>MFKTEFEFPEELKTKLQEHINYFPKKRQAILLCLHEIQNYYGYIPPESLKPLADMLELPLNHVEGVVAFYDMFDREDKAKYRIRVCVSIVCHLMGTNKLLKALENILGIKPGEVTPDGKFKIVPVQCLSACSEAPVFMVNDDEYKFESEVQLNEILSRYT[2x];>[2x]MRSYPAIPRIYAETTLNMLLKRAKKPRVHSIDEYLKDGGYQALEKALNMSPEEIIDWVDKSTLRGRGGAGFPTGKKWKFAVQNPGPRYFICNADESEPGTFKDRIIIERDPHLLIEGIIISSYAIGANEAYIYIRGEYPAGYYILRDAIEEAKKKGFLGKNILGSGFDLEIYVARGAGAYICGEETALIESLEGKRGHPRLKPPYPVQKGLWGKPTVVNNVETIANVPFIISMGWEEYRYIGPSDYAGPKLFPVSGKVKKPGVYELPMNTTLREVIFKYAGGTLGNKKVKAVFSGALDCFSSEELDIPMDYSPLGFGGTGTVIVLTEEDDIVEAALKIAEFYEHETCGQCTPCRVGCYEQANLLEKIYKGEATEQDWEGFDFVNRNIQPTSICGLGAVAGRLIRQTLEKFPEEWE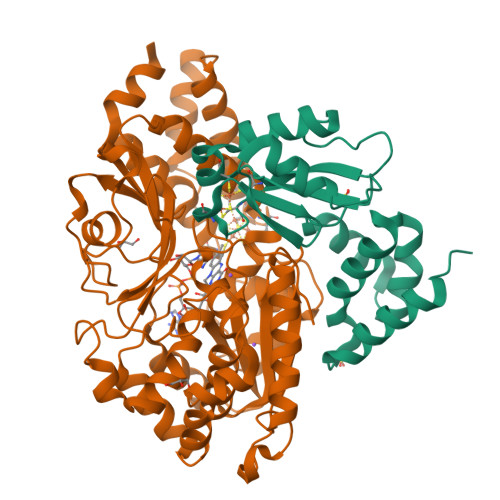KYRKKSASLPLAGHHHHHH>[5x]GPHMSAFEEKAIEKVDDLLESYMGIRDTELAATMVELGKDKRNPDELAEALDERLGDFAFPDEFVFDVWGAIGDAKVGRY;>GPGSHDLSKWKYAE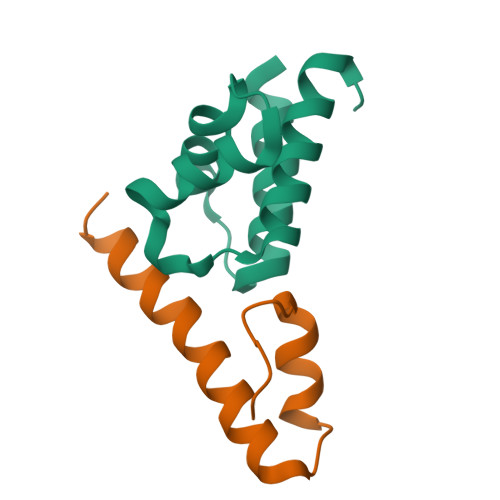LRDTINTSCDIELLAACREEFHRRLKVYHAWKSKN[5x]>ARPAFVNKLWSMVNDKSNEKFIHWSTSGESIVVPNRERFVQEVLPKYFKHSNFASFVRQLNMYGWHKVQDVKSGSMLSNNDS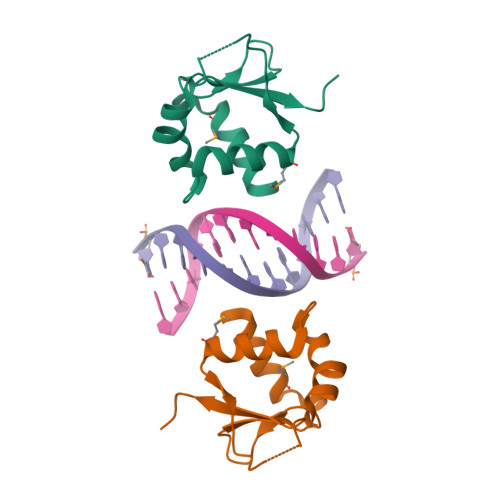RWEFENERHA[2x]>MKWDEIGKNIAKEIEKEILPYFGRKDKSYVVGTSPSGDETEIFDKISEDIALKYLKSLNVNIVSEELGVIDNSSEWTVVIDPIDGSFNFINGIPFFAFCFGVFKNNEPYYGLTYEFLTKSFYEAYKGKGAYLNGRKIKVKDFNPNNIVISYYPSKKIDLEKLRNKVKRVRIFGA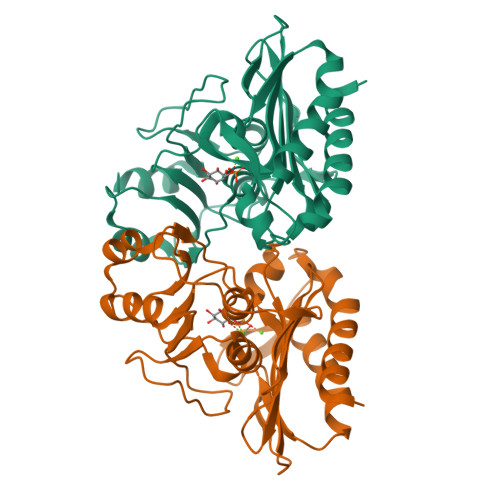FGLEMCYVAKGTLDAVFDVRPKVRAVDIASSYIICKEAGALITDENGDELKFDLNATDRLNIIVANSKEMLDIILDLL[2x]> MGHHHHHHGSLVPRGSYDYLFKVVLIGDSGVGKSNLLSRFTRNEFNLESKST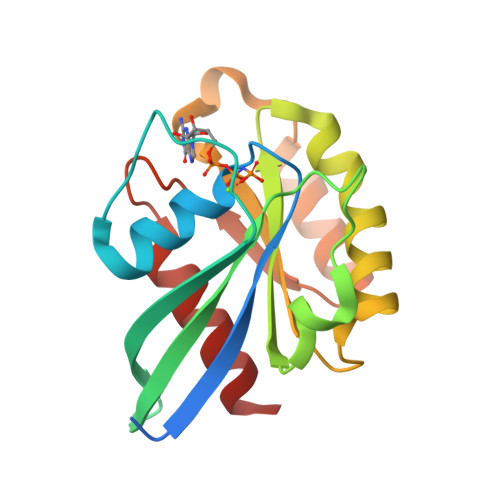IGVEFATRSIQVDGKTIKAQIWDTAGQERYRAITSAYYRGAVGALLVYDIAKHLTYENVERWLKELRDHADSNIVIMLVGNKSDLRHLRAVPTDEARAFAEKNGLSFIETSALDSTNVEAAFQTILTEIYRI(9R,10R)-9-(S-GLUTATHIONYL)-10-HYDROXY-9,10-DIHYDROPHENANTHRENE | C24 H27 N3 O7 S | 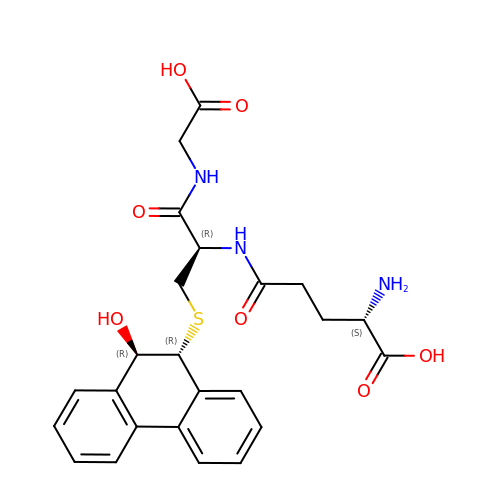JNNIZILNBMPOAC-MOXQZVSFSA-N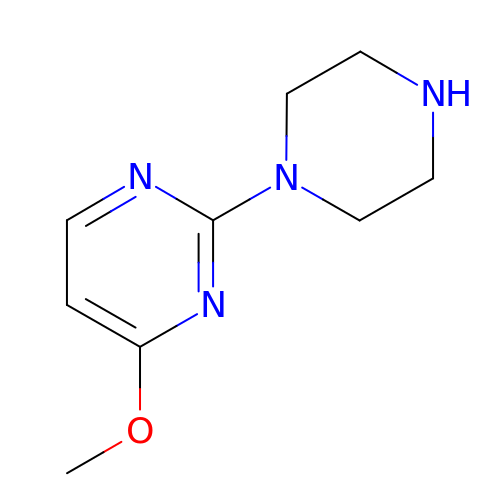4-methoxy-2-(piperazin-1-yl)pyrimidine | C9 H14 N4 O | UWNRWWIRIZDKLH-UHFFFAOYSA-N>[18x]GFFSFIGEAFQGAGDMWRAYTDMKEAGWKDGDKYFHARGNYDAAQRGPGGVWAAEKISDARESFQEFFGRGHEDTMADQEANR

SAA1.1 is an acute phase protein that becomes strongly upregulated during inflammation. Chronic inflammatory conditions, such as tuberculosis, leprosy and rheumatoid arthritis, are risk factors for the development of systemic AA amyloidosis. We report three cryo-EM structures of SAA1.1-derived amyloid fibrils: one that was extracted from the diseased murine tissue and two that were formed from murine SAA1.1 protein in vitro. In vitro and ex vivo fibrils possess parallel cross-β sheets but differ in their overall topologies and fibril protein folds.

The second most abundant fibril morphology (morphology II) represents the majority of the remaining fibrils. Morphology II presents a left-hand twist as demonstrated by platinum side shadowing and transmission electron microscopy (TEM). Using cryo-electron microscopy (cryo-EM) we obtained the structure of morphology II, complementing our previous structure of morphology I22. The 3D map of morphology II achieved a spatial resolution of 3.5 Å, based on the 0.143 Fourier shell correlation (FSC) criterion. Morphology II is polar, C1 symmetrical and consists of three protofilaments (PFs). The PFs are referred to as PF-A, PF-B, and PF-C. The arrangement of PF-A and B in our model is relatively symmetrical and similar to morphology I. The PF-PF interface is formed in both cases by reciprocal ion pairs between residues Asp59 and Arg61. The interactions between PF-B and C also involve complementary charged residues. There are reciprocal interactions between Asp22 and Lys24, as well as a contact of Gly1 (α-amino group) from PF-C with Glu25 (side chain) in PF-B. That is, the packing between PF-B and PF-C is more asymmetrical than that of PF-A and PF-B. Alignment of the fibril proteins reveals only small, if any, conformational differences between the protein folds that construct fibril morphologies I and II.>[24x]PLRLGGNGQLQYWPFSSSDLYNWKNNNPSFSEDPGKLTALIESVLTTHQPTWDDCQQLLG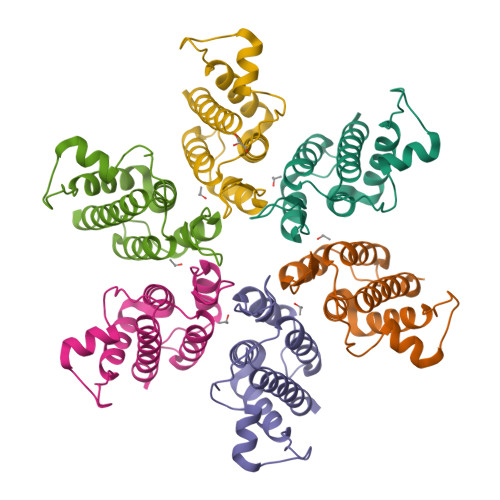TLLTGEEKQRVLLEARKAVRGNDGRPTQLPNEVDAAFPLERPDWDYTTTEGRNHLVLYRQLLLAGLQNAGRSLEHHHHHH> MSSKSEKLEKLRKLQAARNGTSIDDYEGDESDGDRIYDEIDEKEYRARKRQELLHDDFVVDDDGVGYVDRGVEEDWREVDNSSSDEDTGNLASKDSKRKKNIKREKDHQITDMLRTQHSKSTLLAHAKKSQKKSIPIDNFDDILGEFESGEVEKPNILLPSKLRENLNSSPTSEFKSSIKRVNGNDESSHDAGISKKVKIDPDSSTDKYLEIESSPLKLQSRKLRYANDVQDLLDDVENSPVVATKRQNVLQDTLLANPPSAQSLADEEDDEDSDEDIILKRRTMRSVTTTRRVNIDSRSNPSTSPFVTAPGTPIGIKGLTPSKSLQSNTDVATLAVNVKKEDVVDPETDTFQMFWLDYCEVNNTLILFGKVKLKDDNCVSAMVQINGLCRELFFLPREGKTPTDIHEEIIPLLMDKYGLDNIRAKPQKMKYSFELPDIPSESDYLKVLLPYQTPKSSRDTIPSDLSSDTFYHVFGGNSNIFESFVIQNRIMGPCWLDIKGADFNSIRNASHCAVEVSVDKPQNITPTTTKTMPNLRCLSLSIQTLMNPKENKQEIVSITLSAYRNISLDSPIPENIKPDDLCTLVRPPQSTSFPLGLAALAKQKLPGRVRLFNNEKAMLSCFCAMLKVEDPDVIIGHRLQNVYLDVLAHRMHDLNIPTFSSIGRRLRRTWPEKFGRGNSNMNHFFISDICSGRLICDIANEMGQSLTPKCQSWDLSEMYQVTCEKEHKPLDIDYQNPQYQNDVNSMTMALQENITNCMISAEVSYRIQLLTLTKQLTNLAGNAWAQTLGGTRAGRNEYILLHEFSRNGFIVPDKEGNRSRAQKQRQNEENADAPVNSKKAKYQGGLVFEPEKGLHKNYVLVMDFNSLYPSIIQEFNICFTTVDRNKEDIDELPSVPPSEVDQGVLPRLLANLVDRRREVKKVMKTETDPHKRVQCDIRQQALKLTANSMYGCLGYVNSRFYAKPLAMLVTNKGREILMNTRQLAESMNLLVVYGDTDSVMIDTGCDNYADAIKIGLGFKRLVNERYRLLEIDIDNVFKKLLLHAKKKYAALTVNLDKNGNGTTVLEVKGLDMKRREFCPLSRDVSIHVLNTILSDKDPEEALQEVYDYLEDIRIKVETNNIRIDKYKINMKLSKDPKAYPGGKNMPAVQVALRMRKAGRVVKAGSVITFVITKQDEIDNAADTPALSVAERAHALNEVMIKSNNLIPDPQYYLEKQIFAPVERLLERIDSFNVVRLSEALGLDSKKYFRREGGNNNGEDINNLQPLETTITDVERFKDTVTLELSCPSCDKRFPFGGIVSSNYYRVSYNGLQCKHCEQLFTPLQLTSQIEHSIRAHISLYYAGWLQCDDSTCGIVTRQVSVFGKRCLNDGCTGVMRYKYSDKQLYNQLLYFDSLFDCEKNKKQELKPIYLPDDLDYPKEQLTESSIKALTEQNRELMETGRSVVQKYLNDCGRRYVDMTSIFDFMLN;> MTNSVKTNGPSSSDMEYYYKSLYPFKHIFNWLNHSPKPSRDMINREFAMAFRSGAYKRYNSFNSVQDFKAQIEKANPDRFEIGAIYNKPPRERDTLLKSELKALEKELVFDIDMDDYDAFRTCCSGAQVCSKCWKFISLAMKITNTALREDFGYKDFIWVFSGRRGAHCWVSDKRARALTDVQRRNVLDYVNVIRDRNTDKRLALKRPYHPHLARSLEQLKPFFVSIMLEEQNPWEDDQHAIQTLLPALYDKQLIDSLKKYWLDNPRRSSKEKWNDIDQIATSLFKGPKQDSHIIKLRECKEDLVLMTLYPKLDVEVTKQTIHLLKAPFCIHPATGNVCVPIDESFAPEKAPKLIDLQTEMEKNNDVSLTALQPFINQFQAYVSSLLKNELGSVKREREDDDEPASLDF;> MFRQSKRRIASRKNFSSYDDIVKSELDVGNTNAANQIILSSSSSEEEKKLYARLYESKLSFYDLPPQGEITLEQFEIWAIDRLKILLEIESCLSRNKSIKEIETIIKPQFQKLLPFNTESLEDRKKDYYSHFILRLCFCRSKELREKFVRAETFLFKIRFNMLTSTDQTKFVQSLDLPLLQFISNEEKAELSHQLYQTVSASLQFQLNLNEEHQRKQYFQQEKFIKLPFENVIELVGNRLVFLKDGYAYLPQFQQLNLLSNEFASKLNQELIKTYQYLPRLNEDDRLLPILNHLSSGYTIADFNQQKANQFSENVDDEINAQSVWSEEISSNYPLCIKNLMEGLKKNHHLRYYGRQQLSLFLKGIGLSADEALKFWSEAFTRNGNMTMEKFNKEYRYSFRHNYGLEGNRINYKPWDCHTILSKPRPGRGDYHGCPFRDWSHERLSAELRSMKLTQAQIISVLDSCQKGEYTIACTKVFEMTHNSASADLEIGEQTHIAHPNLYFERSRQLQKKQQKLEKEKLFNNGNH;> MSGSIDVITHFGPDADKPEIITALENLTKLHALSVEDLYIKWEQFSNQRRQTHTDLTSKNIDEFKQFLQLQMEKRANQISSSSKVNTSTKKPVIKKSLNSSPLFGLSIPKTPTLKKRKLHGPFSLSDSKQTYNVGSEAETNEKGNSSLKLEFTPGMAEDAVGDSAPLSHAKSSDAKTPGSSTFQTPTTNTPTTSRQNVPAGEILDSLNPENIEISSGNPNVGLLSTEEPSYNQVKVEPFYDAKKYKFRTMRQNLQEASDVLDDQIESFTKIIQNHYKLSPNDFADPTIQSQSEIYAVGRIVPDSPTYDKFLNPESLSLETSRMGGVGRRVRLDLSQVNELSFFLGQIVAFKGKNANGDYFTVNSILPLPYPNSPVSTSQELQEFQANLEGSSLKVIVTCGPYFANDNFSLELLQEFIDSINNEVKPHVLIMFGPFIDITHPLIASGKLPNFPQFKTQPKTLDELFLKLFTPILKTISPHIQTVLIPSTKDAISNHAAYPQASLIRKALQLPKRNFKCMANPSSFQINEIYFGCSNVDTFKDLKEVIKGGTTSSRYRLDRVSEHILQQRRYYPIFPGSIRTRIKPKDVSTKKETNDMESKEEKVYEHISGADLDVSYLGLTEFVGGFSPDIMIIPSELQHFARVVQNVVVINPGRFIRATGNRGSYAQITVQCPDLEDGKLTLVEGEEPVYLHNVWKRARVDLIAS

The eukaryotic polymerase α (Pol α) synthesizes an RNA-DNA hybrid primer of 20–30 nucleotides. Pol α is composed of Pol1, Pol12, Primase 1 (Pri1), and Pri2. Pol1 and Pri1 contain the DNA polymerase and RNA primase activities, respectively. Here we report the cryo-EM analysis of yeast Pol α in the apo, primer initiation, primer elongation, RNA primer hand-off from Pri1 to Pol1, and DNA extension states, revealing a series of very large movements.

We found the apo complex existed in two major conformations and determined their structures to 3.7 Å and 3.8 Å resolution and refer to them here as Apo state conformers I and II, respectively. The apo Pol α-primase is elliptic and measures 150 × 120 × 110 Å. In the apo structure, Pol1 and Pol12 are fully engaged with a buried interface of 202 Å2, in which Pol12 and Pol1-CTD form the “platform”, and Pol1-core tightly binds this platform, such that the OB domain of Pol12 blocks the Pol1-core from binding a polynucleotide substrate from the top, and the Pri2-CTD binds the Pol1-core thumb and palm subdomains from the left side, apparently preventing access of a DNA template to the Pol1-core catalytic site. Due to the small interface with the hinge, Pri1 is partially mobile and fluctuates between two states that are 28.4 Å apart: in apo conformer I, the Pri1-NTD contacts the N-term of Pol1-core, and in apo conformer II, Pri1-NTD connects to the Pol1-core palm instead. The template DNA binding site in Pri1 is exposed, suggesting the apo enzyme is ready to engage the DNA template by the primase but with its polymerase site being autoinhibited. In the Pol α apo state, we observed that Pol1-NTD interacts with Pri1-NTD in ~50% of the particle population, yet the Pri1 EM density is weak and broken. This indicates to us a “transient” nature of the interaction. 1 Pol α fluctuates between apo conformers I and II in the absence of a DNA template, with the Pol1-core catalytic site being blocked by the Pol1-CTD/Pol12 platform and Pri2-CTD and Pri1 moving about. (1) In the apoenzyme resting state (apoenzyme conformers I and II)—before Pol α-primase engages template DNA, it autoinhibits the DNA Pol1-core by sequestering it on the Pol12-Pol1-CTD “platform” but allows the RNA primase Pri1 to rotate about and search for a template (diagram 1). The active site distance is about 70 Å in the apo state.> GSHMASDPKNLKDGQYDIAFKVLKDKTEEISMMNTYVVSPARLTVKDGKKYIAMTLK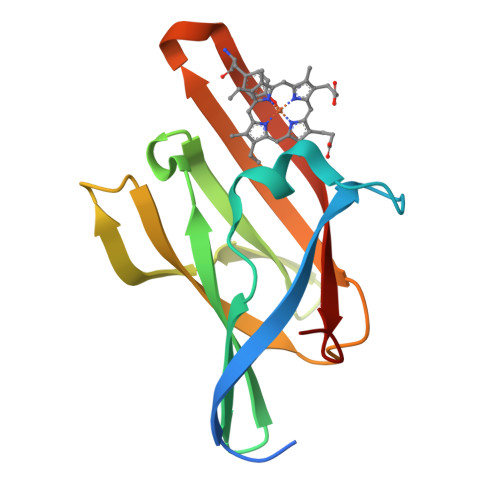NSEWITKFQTEKNGGFADAKVVSEDKAANTRVVEFEANDLFAKLNAKVKVDIDSMNYHHFYDVQIQFDPTKI> MCDSKDNSGVSEKCGKKFTNYPLNTTPTSLNYNLPEISKKFYNLKNKYSRNGYGL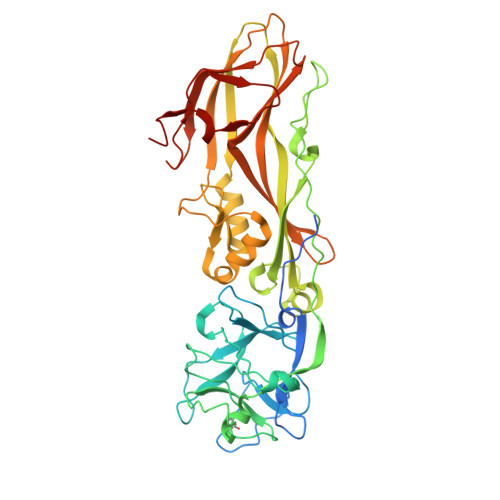SKTEFPSSIENCPSNEYSIMYDNKDPRFLIRFLLDDGRYIIADRDDGEVFDEAPTYLDNNNHPIISRHYTGEERQKFEQVGSGDYITGEQFFQFYTQNKTRVLSNCRALDSRTILLSTAKIFPIYPPASETQLTAFVNSSFYAAAIPQLPQTSLLENIPEPTSLDDSGVLPKDAVRAVKGSALLPCIIVHDPNLNNSDKMKFNTYYLLEYKEYWHQLWSQIIPAHQTVKIQERTGISEVVQNSMIEDLNMYIGADFGMLFYFRSSGFKEQITRGLNRPLSQTTTQLGERVEEMEYYNSNDLDVRYVKYALAREFTLKRVNGEIVKNWVAVDYRLAGIQSYPNAPITNPLTLTKHTIIRCENSYDGHIFKTPLIFKNGEVIVKTNEELIPKINQ>GSEPCVEVVPNITYQCMELNFYKIPDNLPFSTKNLDLSWNPLRHLGSYSFFSFPELQVLDLSRCEIQTIEDGAYQSLSHLSTLILTGNPIQSLALGAFSGLSSLQKLVAVETNLASLENFPIGHLKTLKELNVAHNLIQSFKLPEYFSNLTNLEHLDLSSNKIQSIYCTDLRVLHQMPLLNLSLDLSLNPMNFIQPGAFKEIRLKELALDTNQLKSVPDGIFDRLTSLQKIWLHTNPWDCSCPRIDYLSRWLNKNSQKEQGSAKCSGSGKPVRSIICPT[2x];>[2x]GSQKQYWVCNSSDASISYTYCDKMQYPISINVNPCIELKGSKGLLHIFYIPRRDLKQLYFNLYITVNTMNLPKRKEVICRGS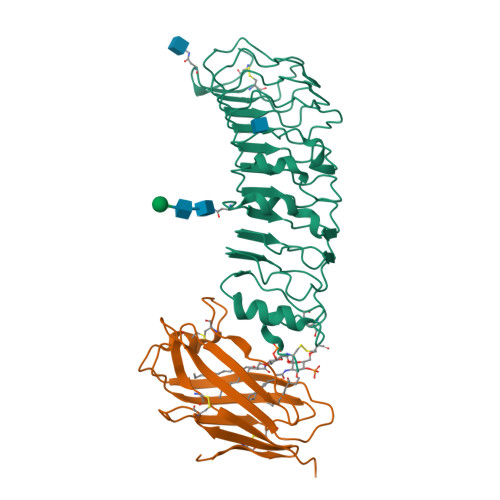DDDYSFCRALKGETVNTTISFSFKGIKFSKGKYKCVVEAISGSPEEMLFCLEFVILHQPN>MDQLQIKDLEMFAYHGLFPSEKELGQKFIVSAILSYDMTKAATDLDLTASVHYGELCQQWTTWFQETSEDLIETVAYKLVERTFESYPLVQEMKLELK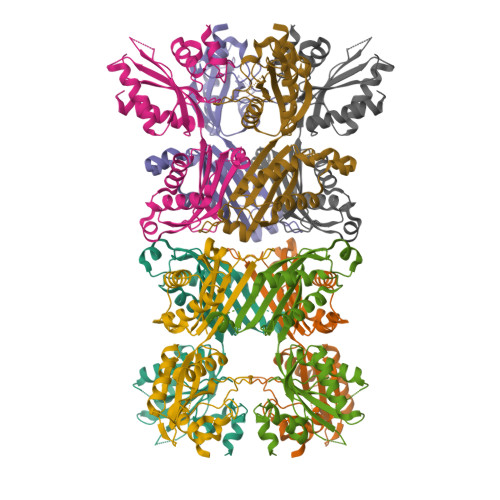KPWAPVHLSLDTCSVTIHRRKQRAFIALGSNMGDKQANLKQAIDKLRARGIHILKESSVLATEPWGGVEQDSFANQVVEVETWLPAQDLLETLLAIESELGRVREVHWGPRLIDLDLLFVEDQILYTDDLILPHPYIAERLFVLESLQEIAPHFIHPILKQPIRNLYDALKK[4x]The acyl-ACP synthetase (termed AasS) of the zoonotic pathogen Vibrio harveyi recycles exogenous fatty acid (eFA), bypassing the requirement of type II fatty acid synthesis (FAS II), a druggable pathway. Very recently, the AasS (533 aa) of V. harveyi was found to feature a large domain at N-terminus (termed AasS_N) that is connected with a compact C-terminal domain by a flexible linker. As expected, a hexamer ring-like overall structure was invariantly formed in all the three types of AasS particles, regardless of a cofactor/inhibitor. Obviously, the pattern of AasS oligomerization is recognized as a trimer of dimers, which mainly relies on two interfaces constituted by the AasS_N domain.

We solved two high-resolution cryo-EM structures of AasS liganded with C10-AMS inhibitor (2.33 Å) and C10-AMP intermediate (2.19 Å) in addition to its apo form (2.53 Å). In addition to the two controls we introduced, (i) AasS alone and (ii) its complex with C10-AMP adenylate, we focused on the complex of AasS liganded with C10-AMS inhibitor. Unlike the two controls that are characterized with a dimension of ‘140x150x80 Å’, the inhibitor-bound AasS architecture is relatively compact, because that its dimension is only confined to ‘130x140x65 Å’. As for apo AasS, its AasS_C domain colored pink, appears in an ‘open’ orientation. Presumably, the AasS monomer adopts an ‘open’ conformation to accept the sequential entry of various substrates ranging from decanoic acid, ATP, to holo-ACP. In brief, the pitcher-like AasS_N domain consists of three β-sheets flanked by α-helices, and provides a centrally-localized cavity for substrate entry. Whereas, the small cap-like AasS_C domain contains one two-stranded and one three-stranded β-sheets surrounded by three α-helices, hovering on top of the AasS_N active sites.

>MNQYVNDPSNYQLLIKNLLFSPVAFNPEQEIVYANHRRHSYKTFHDRVRQFANALTKMGVKKGDTVAVMDYDSHRYLECYFAIPMIGAKLHMINVRLSPEQILYTIDHAEDDIILIHEEFLPILDQIKGRIDTVTRYVVLRDDEECEYERLLEQESTEYNFPDFDENTVATTFYTTGTTGFPKGVFFTHRQLVLHTMGILSTIGTNASQGRLHQGDIYMPITPMFHVHAWGLPYMATMLGVKQVYPGKYVPDVLLNLIEQEKVTFSHCVPTILHLLLSSPKSKAMDFSGWKVVIGGAALPKALCKSALERDIDVFAGYGMSETGPILSIVQLTPEQLELDVDQQAEYRSKTGKKVALVEAYIVDEDMNKLPHDGETAGEIVVRAPWLTPNYYKDNKNSKALWRGGYLHTGDVAHIDDEGFIKITDRVKDMIKISGEWVSSLELEDILHQHQSVSEVAVIGMPHNKWGEVPLALVTLKEDAQVTEKELLGFAKDFINKGILAREALLLKVKIVDEIAKTSVGKVDKKELRKLHL[6x]> LRYT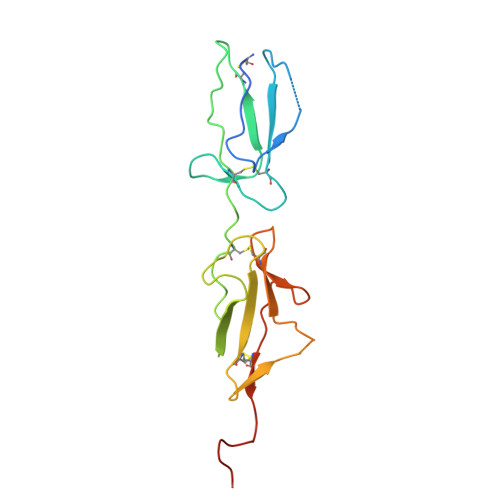TEIIKCPQPKTLDEFTIIQNLQPQYQFRDYFIATCKQGYQLIEGNQVLHSFTAVCQDDGTWHRAMPRCKIKDCGQPRNLPNGDFRYTTTMGVNTYKARIQYYCHEPYYKMQTRAGSRESEQGVYTCTAQGIWKNEQKGEKIPRCLPVCGKPVNPVEQRQR>SEGSDAPNFVLEDTNGKRIELSDLKGKGVFLNFWGTWAEPAKKEFPYMANQYKHFKSQGVEIVAVNVGESKIAVHNFMKSYGVNFPVVLDTDRQVLDAYDVSPLPTTFLI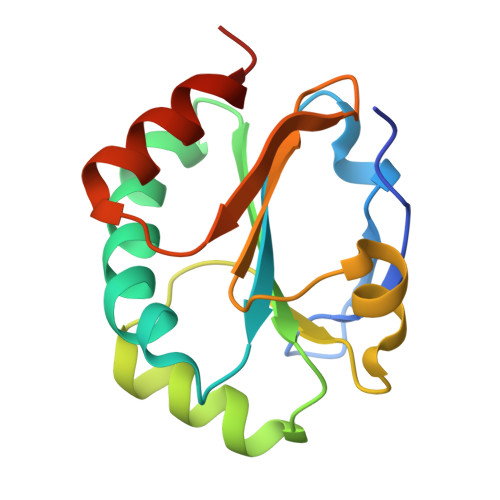NPEGKVVKVVTGTMTESMIHDYMNLIKPGETSG[2x]> Q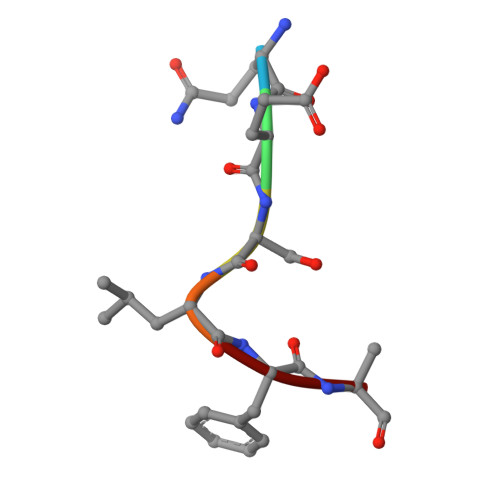ESLFA>[2x]KYLLSPETIEALRKPTFDVWLWEPNEMLSCLEHMYHDLGLVRDFSINPVTLRRWLFCVHDNYRNNPFHNFRHCFCVAQMMYSMV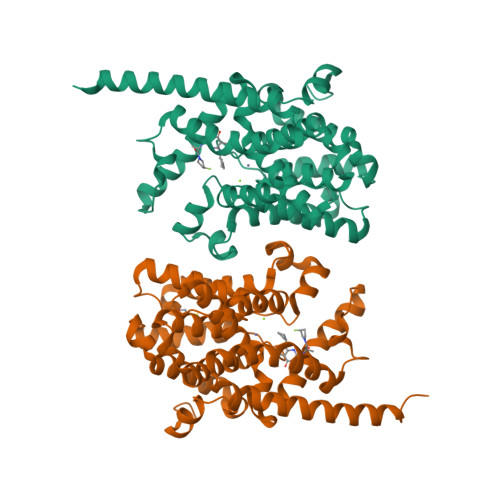WLCSLQEKFSQTDILILMTAAICHDLDHPGYNNTYQINARTELAVRYNDISPLENHHCAVAFQILAEPECNIFSNIPPDGFKQIRQGMITLILATDMARHAEIMDSFKEKMENFDYSNEEHMTLLKMILIKCCDISNEVRPMEVAEPWVDCLLEEYFMQSDREKSEGLPVAPFMDRDKVTKATAQIGFIKFVLIPMFETVTKLFPMVEEIMLQPLWESRDRYEELKRIDDAMKELQKK4-methyl-2-{[2-methyl-6-(methylsulfanyl)phenyl]amino}benzoic 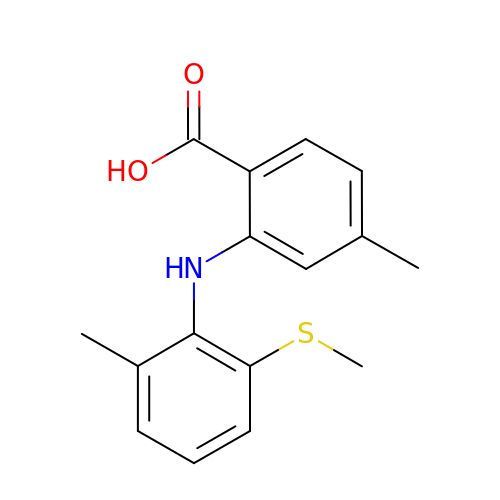acid | C16 H17 N O2 S | WXFNVVGSUPMXIF-UHFFFAOYSA-N>MLERVFIDVDGVKVSLLKGRERKVFYIHSSGSDATQWVNQLTAIGGYAIDLPNHGQSDTVEVNSVDEYAYYASESLKKTVGKAVVVGHSLGGAVAQKLYLRNPEICLALVLVGTGARLRVLPEILEGLKKEPEKAVD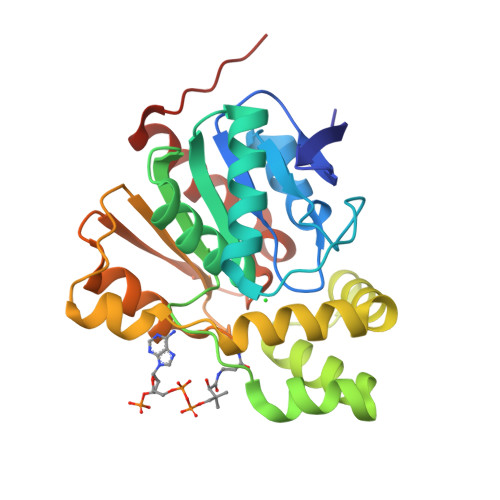LMLSMAFASKGEEYEKKRREFLDRVDVLHLDLSLCDRFDLLEDYRNGKLKIGVPTLVIVGEEDKLTPLKYHEFFHKHIPNSELVVIPGASHMVMLEKHVEFNEALEKFLKKVGVAEVHHHHHH[2x]In this work, we demonstrate these properties using a 9°N DNA polymerase. We show that 3′-esterified dNTP can be incorporated into a template-primer DNA by using MS analysis and X-ray crystallography to validate reaction intermediates and products. We further used structural analyses to examine the incorporation of 3′-NL into DNA.

Before protein crystallization, the incorporation reaction was performed at 4 °C for 16 h with annealed primer-template DNA, dNTP or 3′-NL, and 9°N-I in the presence of Ca2+ (see the Methods section). The DNA with incorporated dAMP is translocated back to the original state, and a divalent ion (Ca2+:1) is near the phosphodiester bond.

>[2x]MILDTDYITENGKPVIRVFKKENGEFKIEYDRTFEPYFYALLKDDSAIEDVKKVTAKRHGTVVKVKRAEKVQKKFLGRPIEVWKLYFNHPQDVPAIRDRIRAHPAVVDIYEYDIPFAKRYLIDKGLIPMEGDEELTMLAFAIATLYHEGEEFGTGPILMISYADGSEARVITWKKIDLPYVDVVSTEKEMIKRFLRVVREKDPDVLITYNGDNFDFAYLKKRCEELGIKFTLGRDGSEPKIQRMGDRFAVEVKGRIHFDLYPVIRRTINLPTYTLEAVYEAVFGKPKEKVYAEEIAQAWESGEGLERVARYSMEDAKVTYELGREFFPMEAQLSRLIGQSLWDVSRSSTGNLVEWFLLRKAYKRNELAPNKPDERELARRRGGYAGGYVKEPERGLWDNIVYLDFRSLYPSIIITHNVSPDTLNREGCKEYDVAPEVGHKFCKDFPGFIPSLLGDLLEERQKIKRKMKATVDPLEKKLLDYRQRLIKILANSFYGYYGYAKARWYCKECAESVTAWGREYIEMVIRELEEKFGFKVLYADTDGLHATIPGADAETVKKKAKEFLKYINPKLPGLLELEYEGFYVRGFFVTKKKYAVIDEEGKITTRGLEIVRRDWSEIAKETQARVLEAILKHGDVEEAVRIVKEVTEKLSKYEVPPEKLVIHEQITRDLRDYKATGPHVAVAKRLAARGVKIRPGTVISYIVLKGSGRIGDRAIPADEFDPTKHRYDAEYYIENQVLPAVERILKAFGYRKEDLRYQKTKQVGLGAWLKVKGKKLEHHHHHH> HHHHHHMPSSV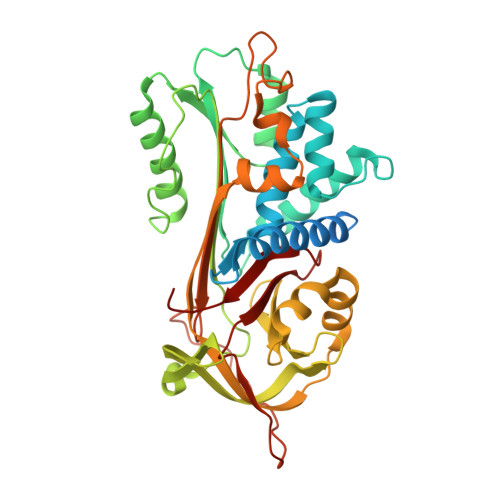SWGILLLAGLCCLVPVSLAEDPQGDAAQKTDTSHHDQDHPTFNKITPNLAEFAFSLYRQLAHQSNSTNIFFSPVSIATAFAMLSLGTKADTHDEILEGLNFNLTEIPEAQIHEGFQELLRTLNQPDSQLQLTTGNGLFLSEGLKLVDKFLEDVKKLYHSEAFTVNFGDTEEAKKQINDYVEKGTQGKIVDLVKELDRDTVFALVNYIFFKGKWERPFEVKDTEEEDFHVDQVTTVKVPMMKRLGMFNIQHCKKLSSWVLLMKYLGNATAIFFLPDEGKLQHLENELTHDIITKFLENEDRRSASLHLPKLSITGTYDLKSVLGQLGITKVFSNGADLSGVTEEAPLKLSKAVHKAVLTIDEKGTEAAGAMFLEAIPMSIPPEVKFNKPFVFLMIEQNTKSPLFMGKVVNPTQK>[4x]MGSDKIH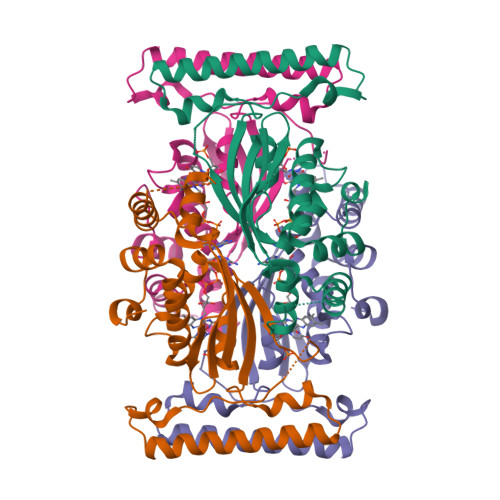HHHHHMKIDILDKGFVELVDVMGNDLSAVRAARVSFDMGLKDEERDRHLIEYLMKHGHETPFEHIVFTFHVKAPIFVARQWFRHRIASYNELSGRYSKLSYEFYIPSPERLEGYKTTIPPERVTEKISEIVDKAYRTYLELIESGVPRRVARIVLPLNLYTRFFWTVNARSLMNFLNLRADSHAQWEIQQYALAIARIFKEKCPWTFEAFLKYAYKGDILKEVQV>MSSKYAVKLKTDFDNPRWIKRHKHMFDFLDINGNGKITLDEIVSKASDDICAKLEATPEQTKRFQVCVEAFFRGCGMEYGKEIAFPQFLDGWKQLATSELKKWARNEPTLIREWGDAVFDIFDKDGSGTITLDEWKAYGKISGISPSQEDCEATFRHCDLDNSGDLDVDEMTRQHLGFWYTLDPEADGLYGNGVP[2x]

Hydromedusan photoproteins responsible for the bioluminescence of a variety of marine jellyfish and hydroids are a unique biochemical system recognized as a stable enzyme-substrate complex consisting of apoprotein and preoxygenated coelenterazine, which is tightly bound in the protein inner cavity. The binding of calcium ions to the photoprotein molecule initiates decarboxylation of 2-hydroperoxycoelenterazine yielding a protein-bound product, coelenteramide, in an excited state. All of them exhibited compact globular structures formed by N- and C-terminal domains within the inner cavity of which the 2-hydroperoxycoelenterazine molecule is disposed. The third His-Trp-Tyr triad is located close to the N1 atom of 2-hydroperoxycoelenterazine but additionally includes a water molecule.

To elucidate the structural basis of the influence of mutations on the bioluminescent properties of the photoproteins, we have also determined the crystal structure of the OL_H64F mutant in conformation before the bioluminescence reaction. The crystal structure of the OL_H64F mutant contains two photoprotein molecules per asymmetric unit. The final model comprises two protein chains (A, B) consisting of 195 and 194 amino acid residues, correspondingly, two 2-hydroperoxycoelenterazine molecules, and 264 molecules of solvent. The OL_H64F mutant, similar to the wild-type photoproteins and their various mutants, is a globular molecule with the radius of ~25 Å. The electron densities detected at the Ca2+-binding loop I in both protein chains A and B (residues 29–37) are conditioned by the bound Na+, just as it was found in the wild-type obelin and Ca2+-discharged obelin-v. Although the coordination geometry is typical for both calcium and sodium ions, no calcium was added to the crystallization solution and hence the ion was recognized as sodium. Thus, the comparison of the OL_H64F mutant structure with those of the wild-type obelin and the OL_Y138F mutant certainly evidences that the substitution of His to Phe does not change the overall structure of this mutant. As expected, similar to the OL_Y138F mutant, the main changes in the substrate-binding cavity of the OL_H64F mutant occur near the N1 atom of the 2-hydroperoxy adduct of coelenterazine. The appearance of the hydrophobic side chain of Phe instead of the hydrophilic chain of His hinders the access of the water molecules in this part of the substrate-binding cavity but does not influence the hydrogen bond between Tyr138 and the N1 atom of the substrate. It should be noted that Phe is found in the same position as His in the wild-type obelin and the OL_Y138F mutant, i.e., the side chain of Phe does not drastically disturb the structure of this part of the inner cavity.>[4x]MSDIGDWFRSIPAITRYWFAATVAVPLVGKLGLISPAYLFLWPEAFLYRFQIWRPITATFYFPVGPGTGFLYLVNLYFLYQYSTRLETGAFDGRPADYLFMLL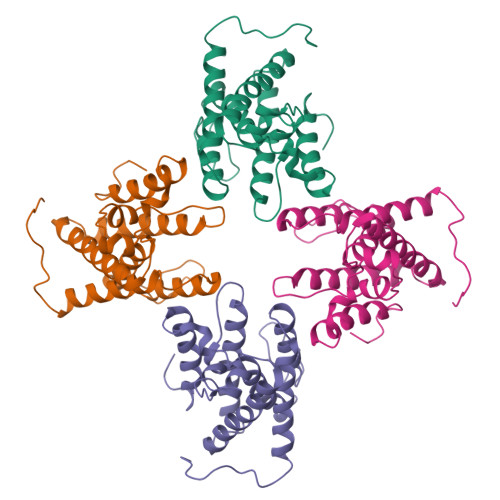FNWICIVITGLAMDMQLLMIPLIMSVLYVWAQLNRDMIVSFWFGTRFKACYLPWVILGFNYIIGGSVINELIGNLVGHLYFFLMFRYPMDLGGRNFLSTPQFLYRWLPSRRGGVSGFGVPPASMRRAADQNGGGGRHNWGQGFRLGDQ>[2x]GTHSLKYVYTGVSRGIDFPEFTAVGMVDDGQFMYFDSNSMKAVPKTEWIRQNEGADYWDRQTQVLIGAHQVFKDSIQIVMERFNQSKGVHTWQNMYGCELNDDGTTQG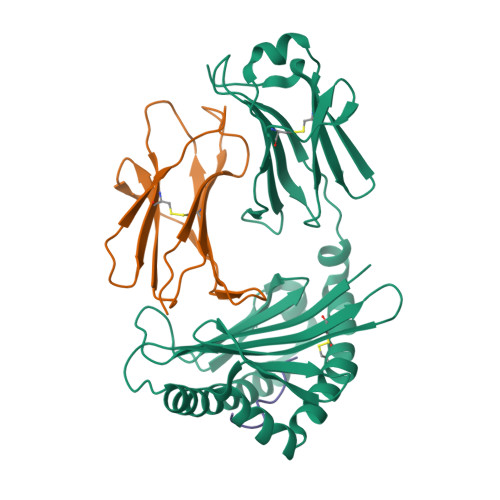FYQYAYDGEDFVSLDKNTLTWTAANPQAVITKHKWEALAVAEQNKGYLENTCIEWLKKYVAYGKDTLERKVSPQVSLLQKDPSSPVTCHATGFYPSGVTITWQKNGQDHDEDVDLGELLPNEDGSFQRMSTLNVGPDEWKNNRFSCVVEHQDKTIRKTEDDIITNFD;>[2x]MRQSDPKVQVYSRNPGEYGKANVLICYVSGFHPPDITIQLLKNGVEIPGSTQTDLAFEEGWQFHLTKYVDFLPQPGEEYTCRVRHMSSPTKSYTWEPDM;>FANFCLMMI[2x]> MTPMKTYDLIVIGTGPGGYHAAIRAAQLGLKVLAVEAGEVGGVCLNVGCIPTKALLHAAETLHHLKVAEGFGLKAKPEL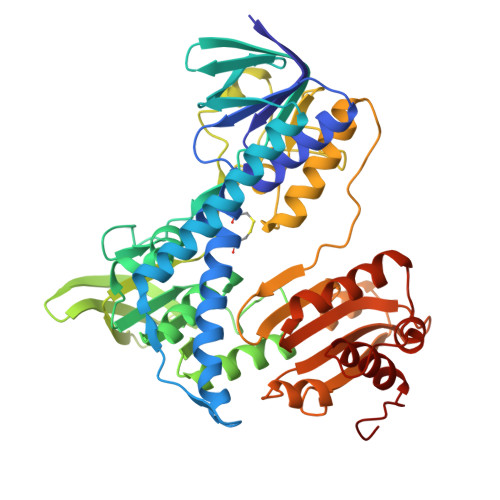DLKKLGGWRDQVVKKLTGGVGTLLKGNGVELLRGFARLVGPKEVEVGGERYGAKSLILATGSEPLELKGFPFGEDVWDSTRALKVEEGLPKRLLVIGGGAVGLELGQVYRRLGAEVTLIEYMPEILPQGDPETAALLRRALEKEGIRVRTKTKAVGYEKKKDGLHVRLEPAEGGEGEEVVVDKVLVAVGRKPRTEGLGLEKAGVKVDERGFIRVNARMETSVPGVYAIGDAARPPLLAHKAMREGLIAAENAAGKDSAFDYQVPSVVYTSPEWAGVGLTEEEAKRAGYKVKVGKFPLAASGRALTLGGAEGMVKVVGDEETDLLLGVFIVGPQAGELIAEAALALEMGATLTDLALTVHPHPTLSESLMEAAEAFHKQAIHILNR> GPGSEFSRHSEKIAIRDFQVGDLVLIILDERHDNYVLFTVSPTLYFLHSESLPALDLKPGEGASGASRRPWVLGKVMEKEYCQAKKAQNRFKVPLGTKFYR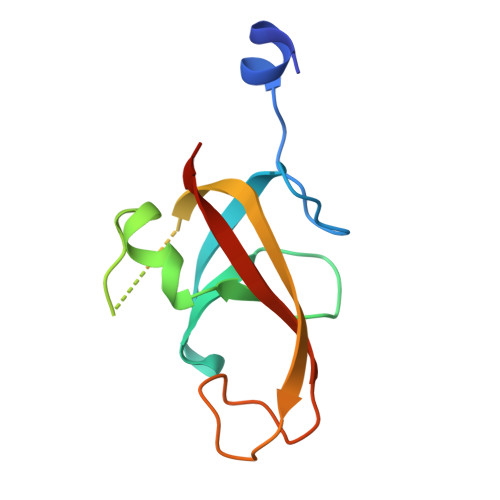VKAVSWNKKV> SAD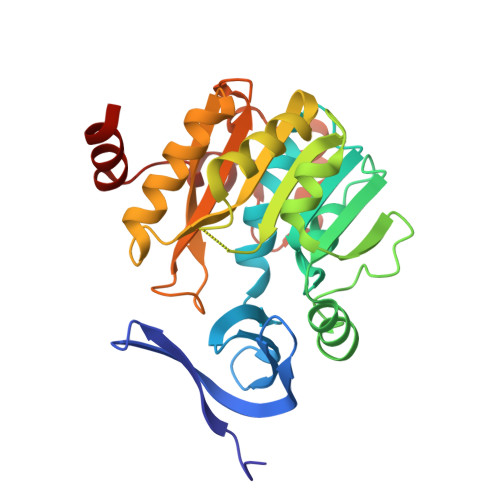APVWIDEVFEDRVRYGLRGQILWEETSPFQKITIVDTEHYGRGLLLDDCWMTAERCEVCYHEYLVHPPLTTAASIARVLVIGGGDGGTVREVLRYAEVEQVDLVEIDGRVVELSQEYLGAIGTAWADPRLNVKIGDGIAFVQTAPDASYDVILVDGSDPAGGLFNREFYENCRRVLKPGGVFASQAESPDSFLAVHLEMIETLSAVFAEAKPYYGWVPMYPSGWWSWLYASDTPGQFQKPQSDRLAAIEPQVEIYNRDIHQAAFAQPNFVRRGLSARQ>MNPVHILAK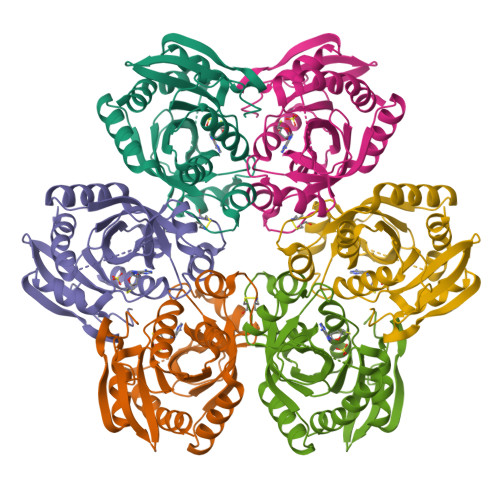KGEVAERVLVVGDPGRARLLSTLLQNPKLTNENRGFLVYTGKYNGETVSIATHGIGGPSIAIVLEELAMLGANVFIRYGTTGALVPYINLGEYIIVTGASYNQGGLFYQYLRDNACVASTPDFELTNKLVTSFSKRNLKYYVGNVFSSDAFYAEDEEFVKKWSSRGNIAVEMECATLFTLSKVKGWKSATVLVVSDNLAKGGIWITKEELEKSVMDGAKAVLDTLTS[3x]Here, we report the cryo-EM structure of the Csm Type III-D complex from S. solfataricus (SsoCsm), which uses CRISPR RNA to bind target RNA molecules, activating the Cas10 subunit for antiviral defence. Type III CRISPR effectors use their crRNA guide to bind cognate RNA molecules, which typically arise from mobile genetic elements (MGE) such as viruses that have previously been encountered by the CRISPR system. This binding activates the Cas10 subunit, which in different species harbours an HD nuclease domain for ssDNA cleavage, a cyclase domain for cyclic nucleotide synthesis, or a combination of both (reviewed in (Tamulaitis et al., 2017)). Type III CRISPR effectors are evolutionary related to type I systems and both share a CRISPR RNA (crRNA) binding “backbone” made up of Cas7 subunits.

The structure of the SsoCsm complex bound to a 48 ​nt crRNA shows its architecture in unprecedented detail. We solved the SsoCsm structure at a final overall resolution of 3.52 ​Å. As the complex was purified from the native host, the bound crRNA is heterogeneous, being sampled from the over 200 spacers present in S. solfataricus P1 (Rouillon et al., 2013; Sokolowski et al., 2014), so the 40 ​nt of the spacer have been modelled as uracils. Overall, the structure is reminiscent of that of other Csm and Cmr complexes (some examples are shown in Fig. 1A), formed of two intertwined helical filaments of multiple stacked subunits wrapping around the crRNA, although SsoCsm is the tallest. Examination of the foot of the complex shows that there is almost no protein:RNA interaction for the Cas10 subunit, while Cas5 makes tight contacts with the guide RNA molecule. The final nucleotide of the 5′ handle, G8 (sometimes also known as position −1 to discriminate between the handle (−8 to −1) and spacer (1 to X) regions of the crRNA), is flipped, as seen in other type III complexes such as SisCmr (Sofos et al., 2020). The remainder of the crRNA adopts a regular pattern with every sixth nucleotide adopting a flipped orientation. Previous studies showed that SsoCsm is unusual in not cleaving at one of the flipped sites, generating a spacing of 12, 6, 6, 6 between sites (Zhang et al., 2016). The missed cleavage corresponds to the Cas7b subunit (1432; chain N in the PDB file, Fig. 3C and D), while subunits competent for RNA cleavage are Cas7a (1430, chain L in the coordinates file), Cas7c (1425, chains F and G) and Cas7d (1426, chains H and I). Analysis of the structure reveals conformational flexibility that most likely relate to target RNA capture and Cas10 activation.

>MRVKHYIQREFNYSVSSQDLLDIATRIAISAIKPKPKSNKPEPYVDSSTINSLLSFLQSRRNVNELLLYIMRQAGRDEIDEETGKLLLASLKDRELKDAVNLLGYVKWVYDTLTGLKVNYNNVKGVKTFKELVNILSKV[5x];>[2x]MSCMDLDVITTVVKIEGKLRNETLLRVGKGKTQDFAEATDNPIIKYRDRPLIPGSSLKGAFRSLVESYTKSLNDSKYYVCDLDDNSCVSCEEKKKDNGIVEGRYCIPCILFGFKDLASRVYILDAIAEKYSISQRTMVAINRVFGGQMPGHLYTLDYVDPGSEFSFMMMIYNLNLIEGEKDWKAKSVEALKFLLATLVREGIFVGARKSVGYGLIKLVDAKVSLYKAPDHLVSPVIVKKLEEVIGTNG;>MVNYTFIDKRVIKRTTMIEGDVETVSPLKIGGGKDNFDPSSLAKDSILKDVEGRPIIPGSSWKGIFRSTGERILRLRNIEVCSGIGKDYCLNNNRKERDFNSALKENVDQALEIFWDYTCLNCKVFGTMSVIGAVRFLDSLPISYSLNTRSMIAISRTEGAVARRALVTVEYVDVGSKFSFKMMGYNLPNYAIGYLITIMKNIHDGFTQVGGHKSRGFGFVKFGKVKFTDLGEKRIGDEDIQVKDVGDLVEGNGDEFFGRMKPFMEAFNNAKIPYPKK[2x];> RSPIRRSNYTPRNEKGLEGVIELQLNVVSDYLHVGSGKYDVEVMRSVSDVKRLVEDYLSGGNKRIPNNVDQYFSMVAFLMVRNKDNVVIPGSTIKGMVRSRLELSVPGSCYIVTGHSTSSSAVYKRIFNPDPNRGSDRFDVNKFPQVCPVCDLLGNMGLASRVSLSDFVMTSGKVDYVNVKGRDYEVVTKGSIFAGKVLYKSLKPVEIGMLLYGFGFVKDCNGSKVMLLGRFKFSDKRFGRVKFSLKTPIADCNKLVSDFVKQFNPRYINEE;> MIRGKLLLPEKKVVFINESEVQSLRKDVVDALKVFSSLACELADNNETKATNIFADLISMIYKLPMLISYVPSDKLSTPHEYFFAYIVFRHLVEDSMPSNDIAKLLEILEEKKRDEIKEVLDYARTLRKIYEKLLYVPADTRPGYNFTSLASHLQLSSILVWLLQKGSVDLNYLRISALLHDIGKLFNPTNHVSESIKILDEVIEGSECLKTNLSRVKSLVEQHHAPLETILNDADRLAASTDRFSEIVKGALNNTKIGECYSLCYGRDVRTKECMECLEEYGEETYSEESKRLYDVISNSVVSQKVEGNAIGYLVYIDFPGIQRFITSFPKLREMSFASFLVDFVTSIYSFIVLDQAYYERTGKKSRIPAEALLSGYGGHSYIIVRSDFGSKDEVKAWLESVSSSALSKLGIRLDVKVADFAYENYVRNYKEVYEDMMSKSYERYLIRDEGKVYSYGLHRVCDNCGIRPAVNRSDDGEYLCETCNLVRDLSKNRGFIAKYKSKYTLYEEQRIEISPKEDIKFKLDKNQDPTSYAMEIIAGYRTTSDSRYIALIKADGNNAGKIFGNTVTFSEYVDKSFRLDFGVKKMFYDTLLDIMRASSDESIKKDLVSRILLGVLYLGGDDIMLLSPSAIAVPFAVKMFKRSLEYTGFTFKVGIISVKPDHPVQFAYGAVNALMEESKIHTGEKSSIGVLVFSSTLASEGVVKSDLKNYRKEKESFLVVSNDVDDVERLLNLMELDDFGKLMELYWNPEEGRKVIRDKIRSLERFVNYADTHDFYNTLAYLIRSKAKSEENSLIKRIIDLTIKGRDDFVFPLYDYYFILKSIRVGI;> MIPIKVSMRNLSSLTIAGGSTISSIDIPLNPLGVPPSTIKGTMRTAVHNLLPNGYTSCGEVEPESIREAHKNGVCDVCKLFGYPDSLTGCFTIDVSKTDYRTSYITRVSIDDKTQRAKEGSLFTQQIILPNSDISFTVYYNCNDERLFKLLLYSILDLRYWRLGRNTMIDVKVNNVEEICKSVKCDEEINGILNQLSRYLWE;> MILIKLKVKGYITTQMRRIRNYYFSITNYIPSTTLRGAILAEYYNQTGKIDENFYVSPAYPIKTAPAHYFSPAKERKGDEFIEVKRILEKKEKEFEANKPIEEIMKLEIDGKHPKPKIGSLITYEGETDKENKYREFSSKSIIQMHVAIDKTSISSYKGMLFAYEYKEFDEMWAIASDSEVIDTVKRIKIGRGKNRGNKVVDVEKVREVSLDQSKGLLYCLSPCIGSLFGKTFFKAKYIIGDKSIYSGWFTVDSFSGQKPVFETLREGSLVYVESFSNEKSLMPAGLNFMLRISDLSSIL;> MVIQVFRLNFRLRTGFRVGGGQEVGDNVIRQLRIGVEGVMIPASSWKGMFRRVSEIVLNSEDHFEEHSKKEVDTRTINALLKSDEKFRRIAISKVGKEVITQNGINVDKLDSESLSDLRRIYNEYNCPIERLYGSNYFAGGITISDSVIPNASIMERTHVTIERKSKKASEKHLFSEEIIDAEKIEVKVIVRNEFELWKNSLKLLREIGYFIGGSKSRGIGYIVLDEKESEYAVINNFSETPKFSELKRYLS> MRPEPGGCCCRRTVRANGCVANGEVRNGYVRSSAAAAAAAAAGQIHHVTQNGGLYKRPFNEAFEETPMLVAVLTYVGYGVLTLFGYLRDFLRYWRIEKCHHATEREEQKDFVSLYQDFENFYTRNLYMRIRDNWNRPICSVPGARVDIMERQSHDYNWSFKYTGNIIKGVINMGSYNYLGFARNTGSCQEAAAKVLEEYGAGVCSTRQEIGNLDKHEELEELVARFLGVEAAMAYGMGFATNSMNIPALVGKGCLILSDELNHASLVLGARLSGATIRIFKHNNMQSLEKLLKDAIVYGQPRTRRPWKKILILVEGIYSMEGSIVRLPEVIALKKKYKAYLYLDEAHSIGALGPTGRGVVEYFGLDPEDVDVMMGTFTKSFGASGGYIGGKKELIDYLRTHSHSAVYATSLSPPVVEQIITSMKCIMGQDGTSLGKECVQQLAENTRYFRRRLKEMGFIIYGNEDSPV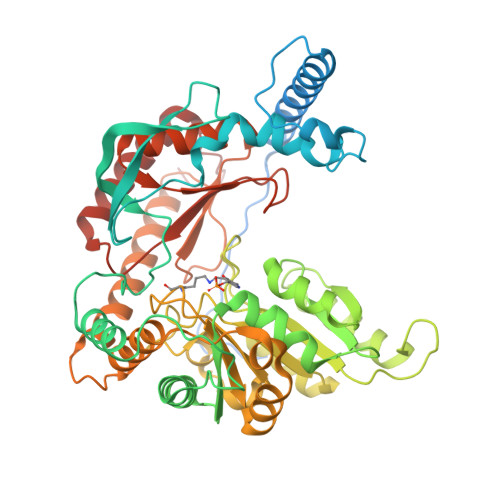VPLMLYMPAKIGAFGREMLKRNIGVVVVGFPATPIIESRARFCLSAAHTKEILDTALKEIDEVGDLLQLKYSRHRL> G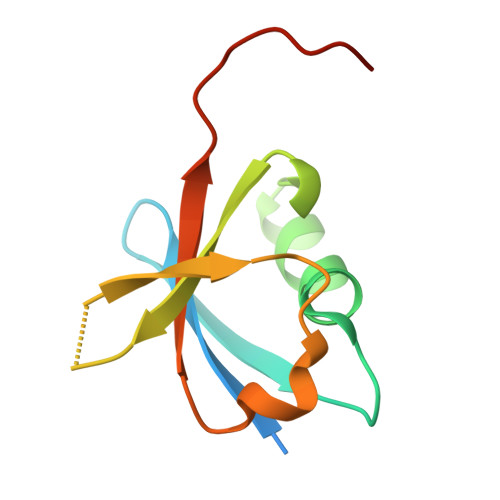PLGSDPSKTSNTIRVFLPNSQRTVVNVRNGMSLHDCLMKALKVRGLQPECCAVYRLQDGEKKPIGWNTDAAWLIGEELQVEFLDHVPLTTHNF>[4x]MNNQKTFKGLRLAALGLVAVAAFTAGCSDVSTELKTPVYKTKLTAEEIRNSAFKPEFPKQYASYERNDETTVMTEYKGSVPFNKNDNVNPLPEGYRHAQPYLKNLWLGYPFMYEYREARGHTYAIQDFLHIDRINRYAEKGGLPATCWNCKTPKMMEWVKESGDGFWAKDVNEFRDKIDMKDHTIGCATCHDPQTMELRITSVPLTDYLVSQGKDPKKLPRNEMRALVCGQCHVEYYFNGPTMGVNKKPVFPWAEGFDPADMYRYYDKHGDLQVKGFEGKFADWTHPASKTPMIKAQHPEYETWINGTHGAAGVTCADCHMSYTRSDDKKKISSH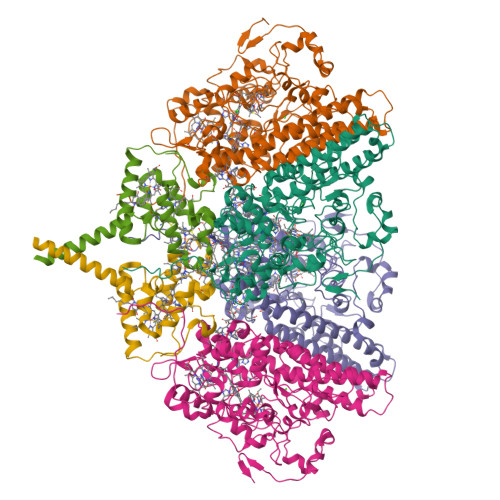WWTSPMKDPEMRACRQCHSDKTPDYLKSRVLFTQKRTFDLLLAAQEVSVKAHEAVRLANEYQGAKAAGYDDLMIQAREMVRKGQFFWDYVSAENSVGFHNPAKALDTLAQSQQFSQKAIDLAMEATQYGIGKDLSGDIKTIVPPILKMNRKLQQDPEFMKTHKWFQYLPVLPKADQVWDGQKRLVSAKQ;>[2x]MSEEKSRNGPARLKLVLGGATLGVVALATVAFGMKYTDQRPFCTSCHIMNPVGVTHKLSGHANISCNDCHAPHNLLAKLPFKAIAGARDVYMNTLGHPGDLILAGMETKEVVNANCKACHTMTNVEVASMEAKKYCTDCHRNVQHMRMKPISTREVADE>MTGMSREEVESLIQEVLEVYPEKARKDRNKHLAVNDPAVTQSKKCIISNKKSQPGLMTIRGCAYAGSKGVVWGPIKDMIHISHGPVGCGQYSRAGRRNYYIGTTGVNAFVTMNFTSDFQEKDIVFGGDKKLAKLIDEVETLFPLNKGISVQSECPIGLIGDDIESVSKVKGAELSKTIVPVRCEGFRGVSQSLGHHIANDAVRDWVLGKRDEDTTFASTPYDVAIIGDYNIGGDAWSSRILLEEMGLRCVAQWSGDGSISEIELTPKVKLNLVHCYRSMNYISRHMEEKYGIPWMEYNFFGPTKTIESLRAIAAKFDESIQKKCEEVIAKYKPEWEAVVAKYRPRLEGKRVMLYIGGLRPRHVIGAYEDLGMEVVGTGYEFAHNDDYDRTMKEMGDSTLLYDDVTGYEFEEFVKRIKPDLIGSGIKEKFIFQKMGIPFREMHSWDYSGPYHGFDGFAIFARDMDMTLNNPCWKKLQAPWEASEGAEKVAASA[2x];>MSQQVDKIKASYPLFLDQDYKDMLAKKRDGFEEKYPQDKIDEVFQWTTTKEYQELNFQREALTVNPAKACQPLGAVLCALGFEKTMPYVHGSQGCVAYFRSYFNRHFREPVSCVSDSMTEDAAVFGGQQNMKDGLQNCKATYKPDMIAVSTTCMAEVIGDDLNAFINNSKKEGFIPDEFPVPFAHTPSFVGSHVTGWDNMFEGIARYFTLKSMDDKVVGSNKKINIVPGFETYLGNFRVIKRMLSEMGVGYSLLSDPEEVLDTPADGQFRMYAGGTTQEEMKDAPNALNTVLLQPWHLEKTKKFVEGTWKHEVPKLNIPMGLDWTDEFLMKVSEISGQPIPASLTKERGRLVDMMTDSHTWLHGKRFALWGDPDFVMGLVKFLLELGCEPVHILCHNGNKRWKKAVDAILAASPYGKNATVYIGKDLWHLRSLVFTDKPDFMIGNSYGKFIQRDTLHKGKEFEVPLIRIGFPIFDRHHLHRSTTLGYEGAMQILTTLVNSILERLDEETRGMQATDYNHDLVR[2x];>MAMRQCAIYGKGGIGKSTTTQNLVAALA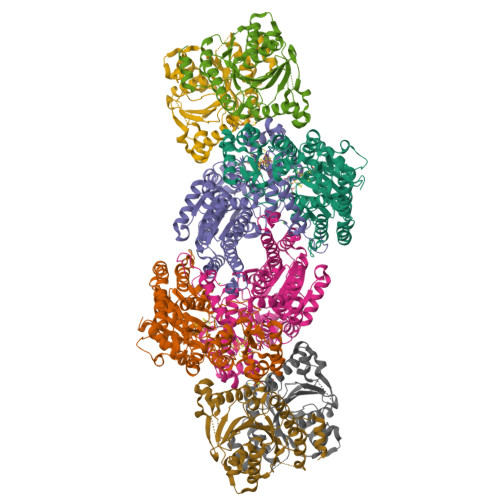EMGKKVMIVGCDPKADSTRLILHSKAQNTIMEMAAEAGTVEDLELEDVLKAGYGGVKCVESGGPEPGVGCAGRGVITAINFLEEEGAYEDDLDFVFYDVGDVVCGGFAMPIRENKAQEIYIVCSGEMMAMYAANNISKGIVKYANSGSVRLGGLICNSRNTDREDELIIALANKLGTQMIHFVPRDNVVQRAEIRRMTVIEYDPKAKQADEYRALARKVVDNKLLVIPNPITMDELEELLMEFGIMEVEDESIVGKTAEEV[4x]> GSHMRPQGATVSLWETVQKWREYRRQCQRSLTEDPPPAT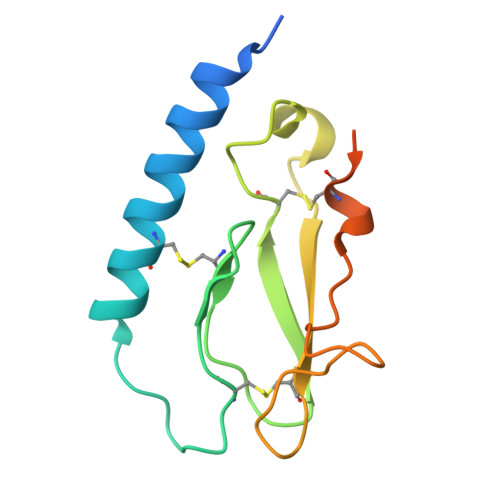DLFCNRTFDEYACWPDGEPGSFVNVSCPWYLPWASSVPQGHVYRFCTAEGLWLQKDNSSLPWRDLSECEESKRGERSSPEEQLLFLY>[2x]MAQKTFKVTADSGIHARPATVLVQTASKYDADVNLEYNGKTVNLK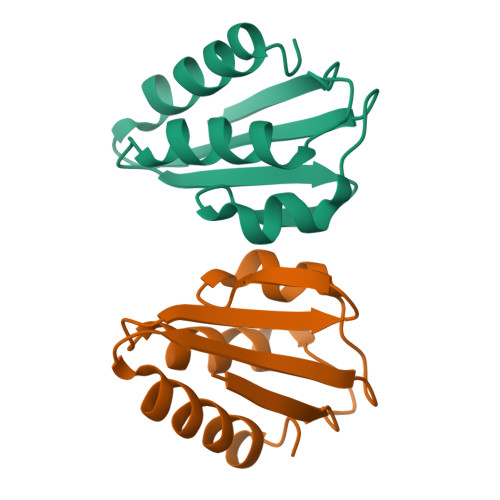DIMGVMSLGIAKGAEITISASGADENDALNALEETMKSEGLGE>GMKRKKKEEEEEKLIVTREFAKRWRDLSGQNHWKGMLQPLDQDLREYIIHYGEMAQAGYDTFNINTESQFAGASIYSRKDFFAKVGLEIAHPYTKYKVTKFIYATSDIHVPESFLLFPISREGWSKESNWMGYVAVTDDQGTALLGRRDIVVSWRGSVQPLEWVEDFEFGLVNAIKIFGERNDQVQIHQGWYSIYMSQDERSPFTKTNARDQVLREVGRLLEKYKDEEVSITICGHSLGAALATLSATDIVANGYNRPKSRPDKSCPVTAFVFASPRVGDSDFRKLFSGLEDIRVLRTRNLPDVIPIYPPIGYSEVGDEFPIDTRKSPYMKSPGNLATFHCLEGYLHGVAGTQGTNKAD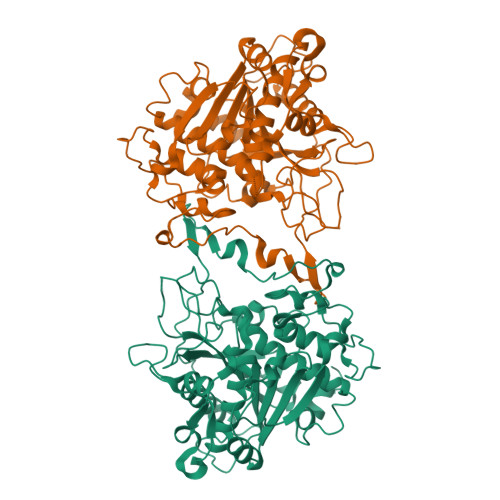LFRLDVERAIGLVNKSVDGLKDECMVPGKWRVLKNKGMAQQDDGSWELVDHEIDDNEDLDF[2x]>GSTGSDKYLTESQFHDKRIAEELRTLLNKSNVYA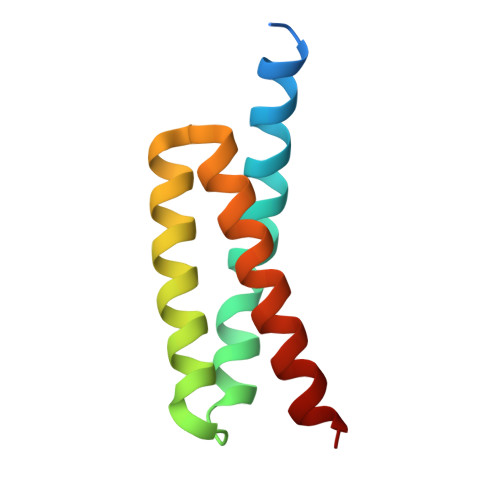LAAGSLNPYYKRTIMMNEYRAKAALKKNDFVSMADAKVALEKIYKEIDEIINR[4x]> LMLHKRNICPIKGCGKNFFSHKYLVQHQRVHSDDRPLKCPWKGCKMTFKWAWSRTEHIRVHTGARPYVCAEPDCGQTF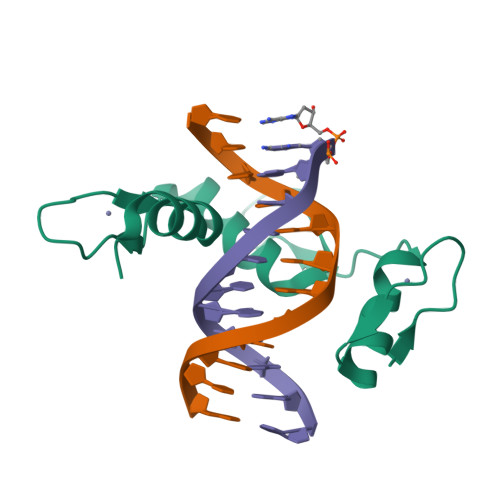RFVSDFSRHKRKTGHSVKKTNKR> MLNFIPKRCPSVSLLFGKRPVQRIEVGQARHQLEIPVET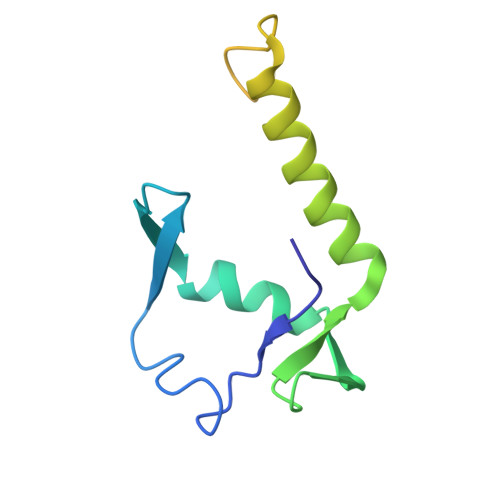IEKIYEGVDSRLEYHNKDYNAMKWKDFMKLKLDAYHLLEASQSETAAKSALSDLNWFSDLADIYSGQQTMAEMDVALKAQGEQKLSYPIQGKNIK>MELRVGNRYRLGRKIGSGSFGDIYLGTDIAAGEEVAIKLECVKTKHPQLHIESKIYKMMQGGVGIPTIRWCGAEGDYNVMVMELLGPSLEDLFNFCSRKFSLKTVLLLADQMISRIEYIHSKNFIHRDVKPDNFLMGLGKKGNLVYIIDFGLAKKYRDARTHQHIPYRENKNLTGTARYASINTHLGIEQSRRDDLESLGYVLMYFNLGSLPWQGLKAATKRQKYERISEKKMSTPIEVLCKGYPSEFATYLNFCRSLRFDDKPDYSYLRQLFRNLFHRQGFSYDYVFDWNMLKFGASRAADDAERERRDREER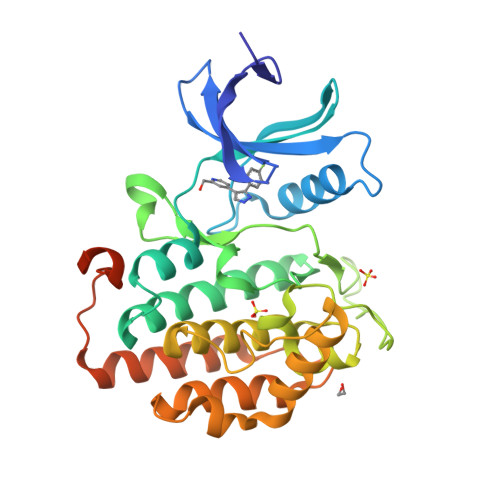LRH[2x]>[2x]MDEERLKEILEELERIIEEVKRLLEKDERLLREFYRRNVTDKEEFRRVIKLDEEVMKRSEELLKRAEELLRELEELIRRIPFSEEIRRELEEILR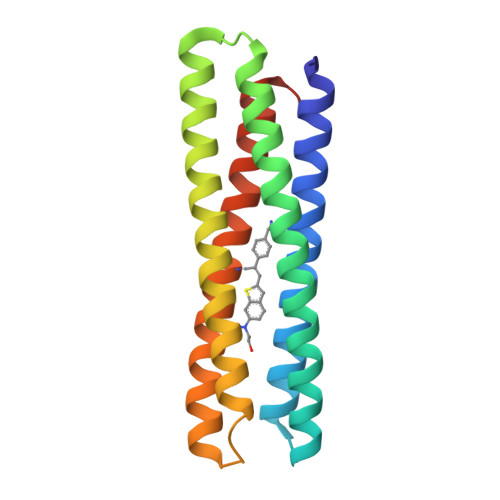RLKELYEEAKRLMEKAKELTKRIKKIDTTDEKTLREWYEIVRELLERAKEIIEEIERLLRRLLEILGLEHHHHHH> MRSSKSPFKRKSHSRETSHDENTSFFHKRTISGSSAHHSRNVSQGAVPSSAPPVSGGNYSHKRNVSRASNSSQTSNFLAEQYERDRKAIINCCFSRPDHKTGEPPNNYITHVRIIEDSKFPSSRPPPDSKLENKKKRLLILSAKPNNAKLIQIHKARENSDGSFQIGRTWQLTELVRVEKDLEISEGFILTMSKKYYWETNSAKERTVFIKSLITLYIQTFEGHVPELVNWDLSLFYLDERSYQRAVITNRPGSVSPIKSPTSNFTTNTTQSVGSVPFSAPTERTRRSETESVNPVSTPASVEYHAGMKSLNKAPYSSNSTLNEVNKRYELEQQQQQEEAELRRLEEQKRLQLQKENEMKRLEEERRIKQEERKRQMELEHQRQLEEEERKRQMELEAKKQMELKRQRQFEEEQRLKKERELLEIQRKQREQETAERLKKEEQEALAKKEEEEKSKRNKVDNESYTQEINGKVDNLLEDLNAVLAEETETTPTMQNGTYVPERSTARAHDQLKKPLNIAKVESLGGSDLNDSISLSDEIAGLNTSNLSGEDQDEKNDLSFEKGDEVRYSNNFEGEAPHVYHEVSIIQEEAPAVSQKLILPEENNESEALIESKEEIKTMENIDDEVLLEILTDINWSIEDDADSMIERIDLRLAETEYLFNQNLLSLQKIGPNIRPYEDKVNDECHRIIPTLSLFLMEMSNFSNDIENVESQDNGLQVESANKKLLWNTLDELLKTVSLDEISLNQLLECPIREKNLPWMENQLNLLLKAFQAIGSDGNEVEYNLREISGLKQRLQFYEKVTKIFLNRIVEEMQKKFSNIRGQDISHDQMIRILTTLLIFSPLILFCKEISQKSYQAIVENWNVSIQPVYMELWTKKISQLQGIDTNDEKMNELSLSQLLNEWDTFRKERKTNDINPVFKNSFSLLTECLQTMRQECIVYQNFVEVFF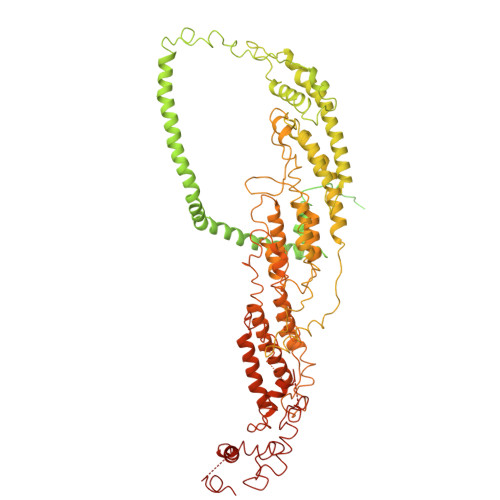HISSKHNFEEYIKHFNDPDAPPILLDTVKVMQSDREAAVIETQLVSRIFQPIVTRLSSYFVELVKAEPTVAPALTFYLENEIKSLESSNHEFLLSAVTRMYTQIKQVWSDNVEEQVLHFERISNATTNGEILPGILDLPVGLKNSEDLFQFAKRSMDIKDTDEGYESIELMNSSFRKLSIAATRSITHKEVNSSINPNLSDTAALNNDYMETISLLVNSNWLTEMLSMLNFNKDGIFDTSLQNVKKVFDVEKESYASFLLRDTMPKLTAFVYGVSNIIENTNNVNMTNPSRWAAYSRQNLENILLAYTSHEIETLVKRLHTHMVNDFGYHQENAINNVLCDKLWSCIQGQTVSLYLKLYTVIDKHYRGTNIRFTKNDIISAFEEYKNA> SNARDMPGHSQEIQTPAIPVNVNLGRSFNQLGIKGSILIYDRNNKKFYEHNAARNSQSFLPASTFKIFNSLVALETGVISNDVAILTWDGMQRQFPTWNQDTNIRQAFRNSTVWFYQVLARKIGHERMEKFIKQVGYGNLQIGTPEQIDRFWLEGPLQITPKQQIEFLQRLHRKELPFSQRTLDLVQDIMIYERTPNYVL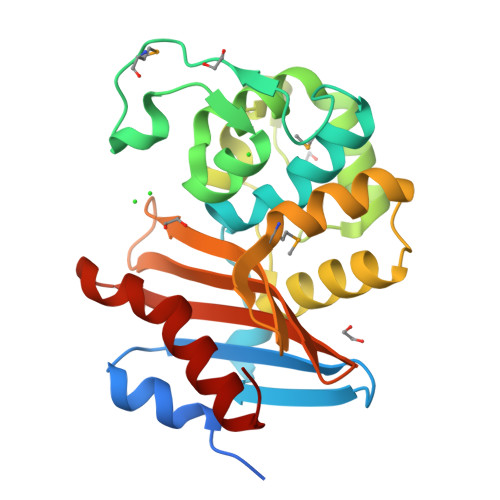RGKTGWAASVTPNIGWFVGYLEQNNNVYFFATNIDIRNNDDAAARIEVTRRSLKALGLL> SACPSGATCGSYTVGGLGSRKQQVRNAGGSSLDLAVAMLQ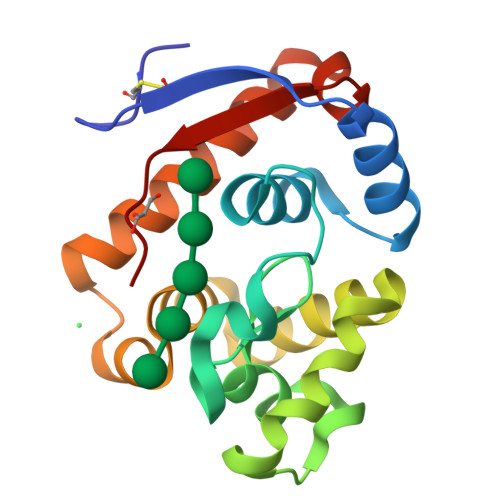TERMDTAYPYGDNKSGDAANFGIFKQNWLMLRSACAQFGGQGAGQYDNGAALNSSLGQDVSCLHQSQSHYGLDAWFAGHRNGASGLSSPNTADIAAYKAAVYWIKAQLDADSANLGNDTRFWVQVPAI>[2x]MNGRRK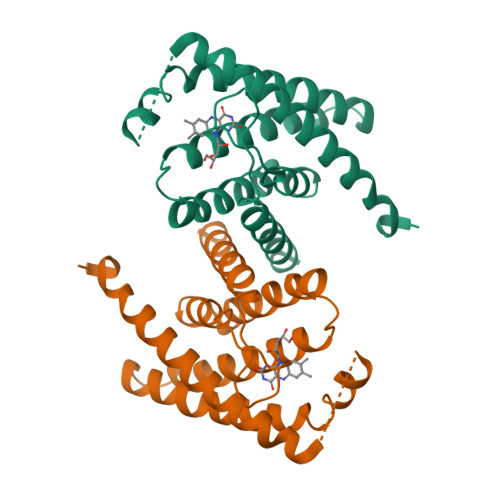LNMQQNKRLITISMLSAIAFVLTFIKFPIPFLPPYLTLDFSDVPSLLATFTFGPVAGIIVALVKNLLNYLFSMGDPVGPFANFLAGASFLLTAYAIYKNKRSTKSLITGLIIATIVMTIVLSILNYFVLLPLYGMIFNLADIANNLKVIIVSGIIPFNIIKGIVISIVFILLYRRLANFLKRI> GSMSATLKDYLNKRVVIIKVDGECLIASLNGFDKNTNLFITNVFNRISKEFICKAQLLRGSEIALVGLIDAEN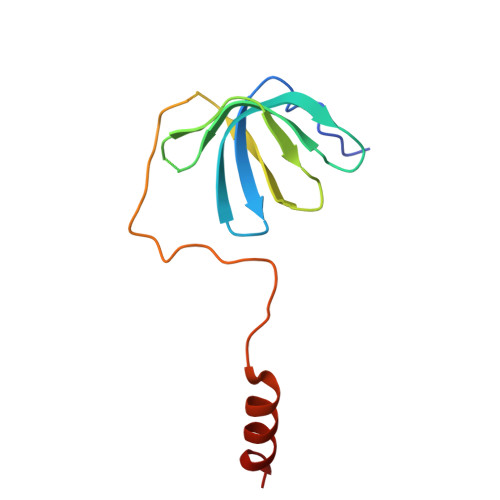DDSLAPIDEKKVPMLKDTKNKIENEHVIWEKVYESKTK> AMADTIVAVELDSYPNTDIGDPSYPHIGIDIKSIRSKSTARWNMQTGKVGTAHISYNSVAKRLSAVVSYSGTSSTTVSYDVDLNNVLPEWVRVGLSATTGLYKETNTILSWSFTSKLKTNSIADANSLHFSFSQFSQNPKDLILQSDATTDSDGNLQLTRVSSDGSPQGSSVGRALFYAPVHIWEKSAVVASFD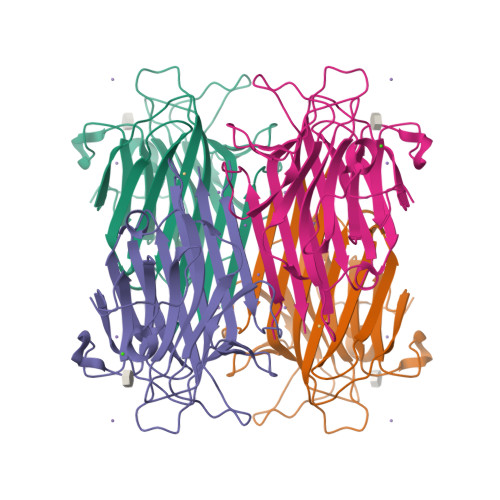ATFTFLIKSPDRDPADGITFFIANTDTSIPSGSGGRLLGLFPDAN> MNVLVPGIDGMVSAGKFEYSGCCPPDFADMDECTLATSYVGLLPSGPLWDRAKYEAITTITATGNCAACWTEDHCPTLVDYAVNVGARLASVIDMTLWPAVRESDPFTAVTSTADWLERFKWVNCFETSCR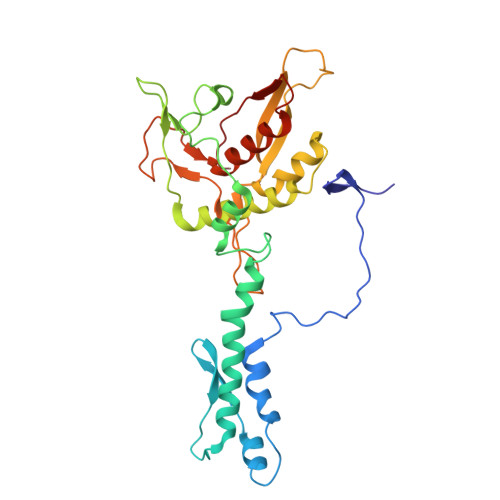SKALGEITPIEYMTECGPVYVAINYPPSIKQAFESALIKSLERLSMGIIKNLASINFVIEPLKVRVVPLDTTNACENETLCVTFEKTSDFFDGVNQNPCGIPSPVAAYIDRDVMQLPSELPKYIWPGHMAAECVVRSLLSHVSRFCVVRTDQTPD>[2x]MSAESVAATPESAGGHIRLTSHSGGVGALPIHWGAPTASERGPVVGTTTNRAHRNVIGTHSGSYSIYRALAVASGALSRHHKADLTDTAPTNIIGPYPQWSQPGKIVSLDPWGATVAEVFAAELAAGHDIRPSIAVTKAHVILPEVMEAIQKGRLHPDGRFL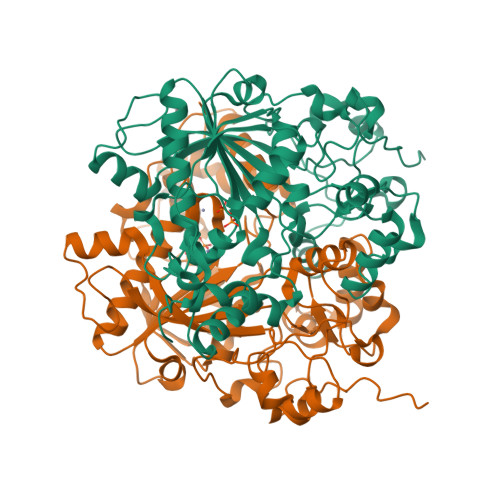LPSGAALVTKAAIEPVWHLPGVAERFHCSETDLRRVLFEETGGMYPELVTRSDLEVFLPPIGGQTVYIFGDARDLADPGVELTARVHDECNGSDVFGSDICTCRPYLTHAIEECIQGAQRGGVGLVAYSRKEGRALGEVTKFLVYNARKRQVGGDTADQYFARTECVAGVQDMRFQEMMPDVLHWLGVRKIHRLVSMSNMKYDAITGSGIEVVERVDLPADLIPADARVEIDAKMAAGYFTPGAVPDADELAKVKGRELDG> QGVNIYNISAGTSVDLAAPVTTGDIVTFFSSALNLNAGAGN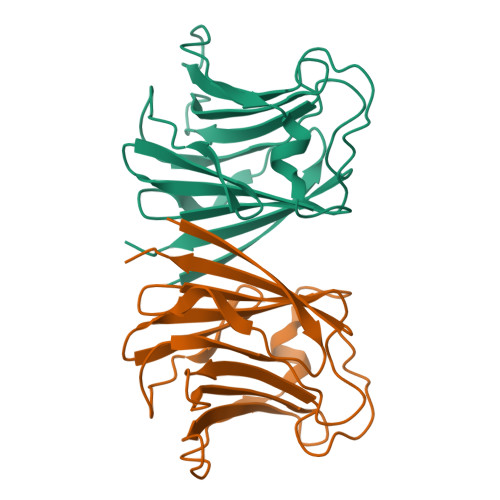PNNTTLNLFAENGAYLLHIAFRLQENVIIFNSRQPDGPWLVEQRVSDVANQFAGIDGKAMVTVFDHGDKYQVVINEKTVIQYTKQISGLTSSLSYNATEETSIFSTVVEAVTYTGLA>GGUCACAGCCC[2x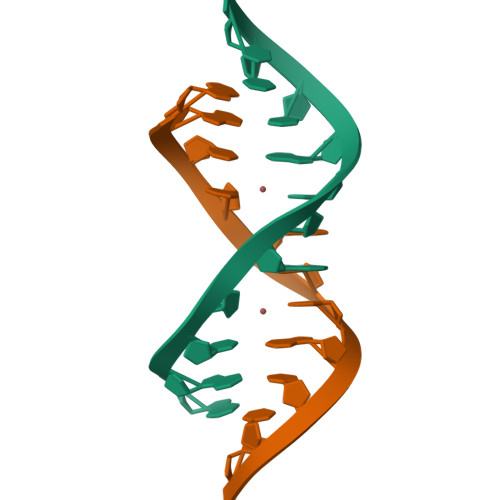]> RTA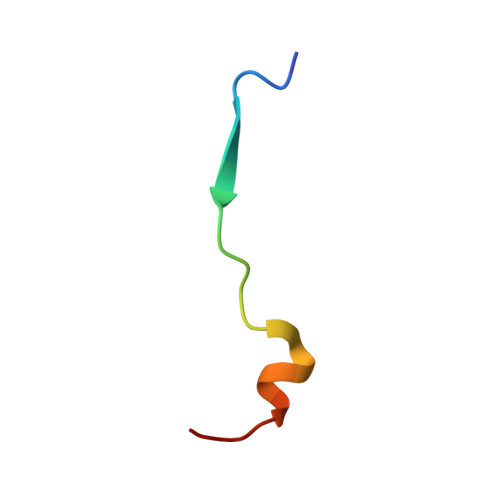NILKPLMSPPSREEIMATLL>[4x]GMRMSSTGEYVPSPSEWIGNQVAQYEASDGAEAGEFDGRPLVILTTVGRKTGALRKTPVMRVEHDGRYAVVASQGGAPTH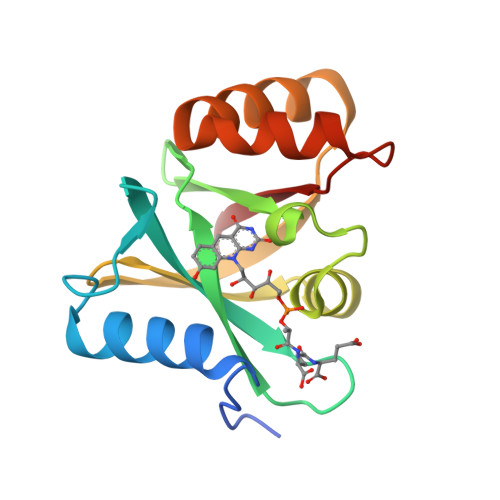PAWYFNLVADPRAQLRDKDAVLSVVARELAGPERAEWWERAVRAYPTYQEYQDNTRRLIPVLLLEPG> MPNPSPPSSSSPVQTLISILRIIPDWSDRTQERGMRQHRTLYDHEKWMHHRSSYRHLRHLLSSLSSRVILSLIPPVIAFTLVAVVIASYNTAVALDLLPGIFPLLRSSSLPYQLTAPALALLLVFRTEASYSRFEEGRKSWTEVIAGANDFARQIISSVETSGDAQLKKALLQYIVAFPVALKCHVIYGSDIARDLQN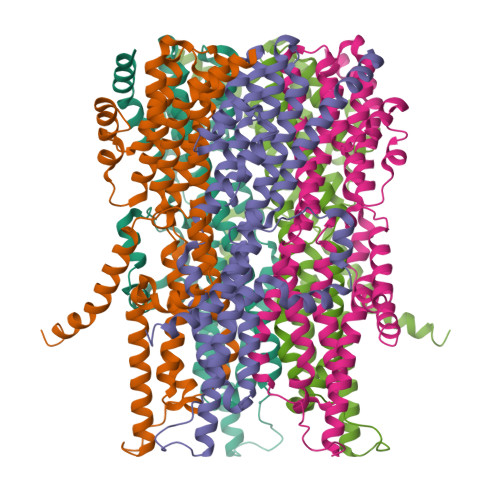LLEVDDLLVVLNSKHRPGCIIQFISRSLQLLKLEESRRIMLQSKISCFHEGIGICEQLIGTPIPLSATRLTSRFLVLWHLTLPIILWDDCHWIVVPATFISAASLFCIEQVGVLIEEPFPMLALDDLCNSVRNNVQEALASEKLIRARLAAKGRIQSEQQFQNGQPRPENLYFQ>SNAMKILQIKPHFRAEIIEPKHVYLLSESSTHALTGELYCQLIPLLNGNYTVDEIINKLQVDPSHIDYALERLQARGYITEAIPQLTPEAVAFWGLLKVEPQVAYQCLQQTQVYVSSVVNLPTQPLITALEEVGIKAINWDGELQEFPPHSLLVVLTDDYLQPQLNKINQIALKANQPWLLIKPVGTILWLGPIFQPQITGCWECLAQRLRVNREVEASVLRQKNSSLQLSPSQELNSSVLQSNGNGVKSEVIECLPPPAAVIPSTLQTALHLATTEIAKWIVKQGVEDTTPFPTLEGKVITFDQRNLDLQTHILSLRPQCPSCGNPNLLTERAFQPLVLSSRKKQFTSDGGHRAFSPDQTVNRYQHLISPITGVVTSLVRASDPNDSLNHTYNAVHSFVIASNIGRMRRYLKHKSSGKGKTDSQSKASGFCEAIERYSGVYQGDEPRISATLAELGEKAIHPARCSLFSSEQYEYREEFNRRGGVFDWIPQPFDETKVIEWTPVWSLTEQTHKYIPTAYCYYGYPLPEDHEFCRANSNGDATGNTLEEAIIQGFFEIVERDSVAIWWYNRLKRPAVDLASFNEPYLLEVQDLYRSNNRDLWVIDITADLDIPTFVAVSYLKDNKHQTILLGFGTHFDPKIAILRAVTEVNQIAFTCDGVEVTKEFVEMREWFKKATIENQPYLVPDSTVPAKVYQDYQQR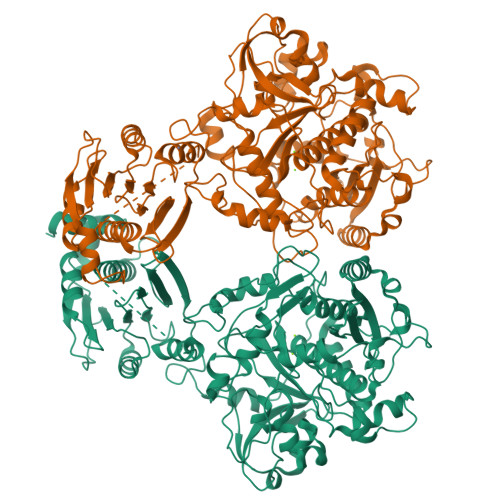WSDDIYEDVMTCVEISKNAGLETLVLDKTRPDIGLNVAKVIVPEMPHYWLRMGAKRIYDVPVKMGWLSTPLTEEQMNPISVPI[2x]>[4x]MPLDPEVRNFLQVYYKANIIDFTKYQFQEIRQKVNELLAKAVPKDPVGETRDMKIKLEDYELPIRIYSPIKRTNNGLVMHFHGGAWILGSIETEDAISRILSNSCECTVISVDYRLAPEYKFPTAVYDCFNAIVWARDNAGELGIDKDKIATFGISAGGNLVAATSLLARDNKLKLTAQVPVVPFVYLDLASKSMNRYRKGYFLDINLPVDYGVKMYI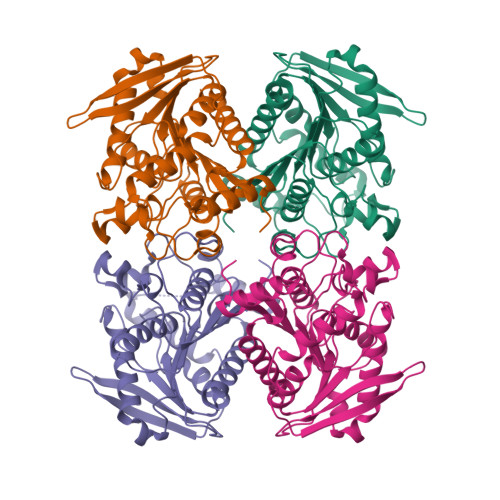RDEKDLYNPLFSPLIAEDLSNLPQAIVVTAEYDPLRDQGEAYAYRLMESGVPTLSFRVNGNVHAFLGSPRTSRQVTVMIGALLKDIFK In contrast, cryo-crystallography has effectively addressed such issues, leading to the seminal success of synchrotron structural biology. In this study, we introduce a pragmatic high-throughput RT data-collection method, Cryo2RT, that takes advantage of the well established workflow for synchrotron cryo-crystallography. The procedure involves crystal cooling in liquid nitrogen (LN2) at the laboratory, shipping to the synchrotron under cryogenic conditions, as is commonly practiced, and thawing the crystals on the goniometer immediately before X-ray data collection. Here, we used endothiapepsin (EP) soaked with four different fragments, thaumatin (Thau) and SARS-CoV-2 3CLpro (3CLpro) as test systems to show that RT structures can be obtained after the cooling/thawing process. Our Cryo2RT method applies to conventional single-crystal data collection and achieves a comparable throughput to cryo-crystallography, enabling high-throughput fragment-based screening at RT: a highly sought-after method in structure-based drug discovery.

Therefore, we set out to perform similar experiments using conventional single crystals mounted with standard cryoloops for three protein targets (EP, Thau and 3CLpro). Cryo2RT was also applied to Thau and 3CLpro cryoloop crystals, yielding high-quality data sets after the cooling/thawing process. In this study, we systematically observed a slightly lower resolution for crystals collected at RT compared with cryo temperature, even though the same dose of a few hundred kilograys was used.

> MAATTCFFFLFPFLLLLTLSRAATFEIVNRCSYTVWAAASKGDAALDAGGRQLNSGESWTINVEPGTNGGKIWARTDCYFDDSGSGICKTGDCGGLLRCKRFGRPPTTLAEFSLNQYGKDYIDISNIKGFNVPMDFSPTTRGCRGVRCAADIVGQCPAKLKAPGGGCNDACTVFQTSEYCCTTGKCGPTEYSRFFKRLCPDAFSYVLDKPTTVTCPGSSNYRVTFCPTALELEDE>MMANRMILNETAWFGRGAVGALTDEVKRRGYQKALIVTDKTLVQCGVVAKVTDKMDAAGLAWAIYDGVVPNPTITVVKEGLGVFQNSGADYLIAIGGGSPQDTCKAIGIISNNPEFADVRSLEGLSPTNKPSVPILAIPTTAGTAAEVTINYVITDEEKRRKFVCVDPHDIPQVAFIDADMMDGMPPALKAATGVDALTHAIEGYITRGAWALTDALHIKAIEIIAGALRGSVAGDKDAGEEMALGQYVAGMGISNVGLGLVHGMAHPLGAFYNTPHGVANAILLPHVMRYNADFTGEKYRDIARVMGVKVEGMSLEEARNAAVEAVFALNRDVGIPPHLRDVGVRKEDIPALA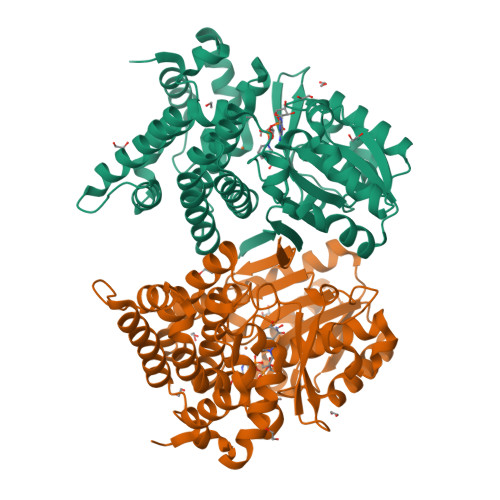QAALDDVCTGGNPREATLEDIVELYHTAWTSHHHHH[2x]Members of glycosyltransferase family 75 (GT75) not only reversibly catalyze the autoglycosylation of a conserved arginine residue with specific NDP-sugars but also exhibit NDP-pyranose mutase activity that reversibly converts specific NDP-pyranose to NDP-furanose. MtdL from deep sea–derived Marinactinospora thermotolerans SCSIO 00652 has been discovered in the antibiotic A201A biosynthetic pathway, generating GDP-L-galactofuranose (L-Galf) from GDP-L-galactopyranose (L-Galp). The MtdL subunit is divided into three regions: the N-terminal region (residues 1–111), the core region (residues 112–291), and the C-terminal region (residues 292–376). The characteristic DXD motif (Asp109-Asp110-Asp111), together with conserved His287, coordinates a Mn2+ ion, which stabilizes the diphosphate of the nucleotide.

Then, the complex structure of MtdL bound to Mn2+ and GDP at 2.1-Å resolution was obtained by cocrystallizing MtdL containing 0.5 mM MnCl2 with GDP, which led to a clear electron density for both the GDP diphosphate moiety and the Mn2+ ion at the active site. In the Mn2+·GDP bound structure, the Mn2+-binding site is formed by Asp111 at the third position of the DXD motif on the loop following β4 and a conserved histidine His287 at the end of β15. This Mn2+ coordination is slightly different from that observed in other GT-A glycosyltransferases, where both aspartates in the DXD motif coordinate to Mn2+ directly. In addition, each phosphate group of GDP coordinates to Mn2+ through a single oxygen atom, as shown in other GT-A enzymes. In the MtdL·Mn2+·GDP structure, the α- and β-phosphates of GDP interact with the side chains of Asp111 and His287 via a Mn2+ ion. In addition, β-phosphate forms hydrogen bonds with the side chains of Gln229, Arg257, His287 and Arg289, while α-phosphate forms hydrogen bonds with the side chain of His292. Structural comparison of GDP-MtdL complexes in the absence and presence of Mn2+ indicated a major conformational change in loop A (residues 288–292), which follows the Mn2+ coordinating His287 on β15. By contrast, loop A displayed two conformations in the Mn2+·GDP bound structure. One is distal from the diphosphate group, similar to that shown without Mn2+, while the other is in the vicinity of the diphosphate. The side chains of Arg289 and His292 on loop A formed new hydrogen bonds with the diphosphate of GDP in the presence of Mn2+.

>[2x]HMSGRDISTAVVVTTISDGGFLDRLAPALRDAGARLIVIPDRNTGPALFAACERHRRLGLDVVCPSVAEQQDLLERLAVPDLIPYHSDNRRNVGYLMAWMEGFDVIVSMDDDNLPTTDDFVERHQVVCQGPRTQPVTASSDGWFNNCALLEVEPTEVFPRGFPFHARPAHAQARTSVCERPADVRINAGLWLGDPDVDAITRLAVRPNALAHSGGSVVLAEGTWCPVNSQNTAVHRDALPAYYFLRMGQPVDGVPMERFGDIFSGYFVQVCAQHLGHAVRFGDPVVEHPRNEHDLLDDLHKEVPAVRLLDDILDHLRDHPLEGGDYLETYESLSYALQEIAERVNGRAWSPDARAFLHRSAHLMRSWTGALRTVAGT>ACGGGSSNSGQPSQESNVKEIDVWAWDPSLKQIAADYEKKTGIKVNLKNVGTNTKEYTQLDNAIEAGSGAPDVAQIEYYALPQYAIKGNLLDITDKTSGYEDFYNPGPWSSVQIDGKVYALPIDAGPMAFFYNKEIFDKAGVDGEKIKTWDDYYEAAKKIHALGDEYYITSDSGDAGFFDSMTWLAGGKPFQTTNNGKDVTINLTGDNGVKEFEKFWQKLLDEKLLDTKTVGWSEDWFKGMQDGTIASLLTGAWMPGNLVNSAPAAAGKWRVALMP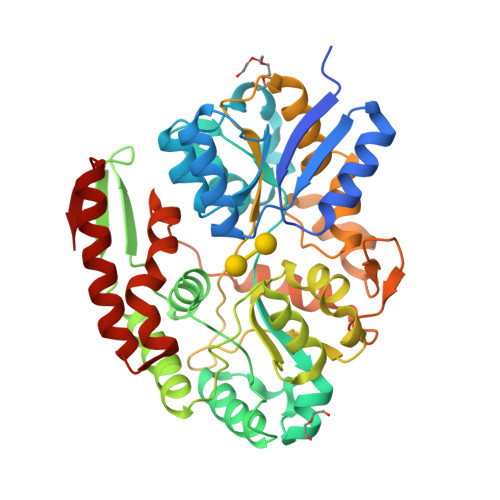TPNGEKANAENGGSSLAVLKSSPKAQAAYDFIEYVAHGDGVKTHVETGAFPADKASLEADYFKNATTIKNSDGKEIDYFGGQKYNEVLAQASADVLTGYQFLPFEVKARGVFGDYLGKSYTGNQPLSEGVAAWQKALIDYGKEQGFTMKE[2x]>MRPYYIAIVGSGPSAFFAAASLLKAADTTEDLDMAVDMLEMLPTPWGLVRSGVAPDHPKIKSISKQFEKTAEDPRFRFFGNVVVGEHVQPGELSERYDAVIYAVGAQSDRMLNIPGEDLPGSIAAVDFVGWYNAHPHFEQVSPDLSGARAVVIGNGNVALDVARILLTDPDVLARTDIADHALESLRPRGIQEVVIVGRRGPLQAAFTTLELRELADLDGVDVVIDPAELDGITDEDAAAVGKVCKQNIKVLRGYADREPRPGHRRMVFRFLTSPIEIKGKRKVERIVLGRNELVSDGSGRVAAKDTGEREELPAQLVVRS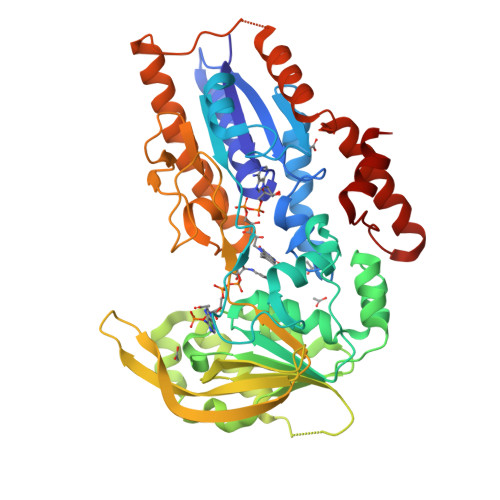VGYRGVPTPGLPFDDQSGTIPNVGGRINGSPNEYVVGWIKRGPTGVIGTNKKDAQDTVDTLIKNLGNAKEGAECKSFPEDHADQVADWLAARQPKLVTSAHWQVIDAFERAAGEPHGRPRVKLASLAELLRIGLG[2x]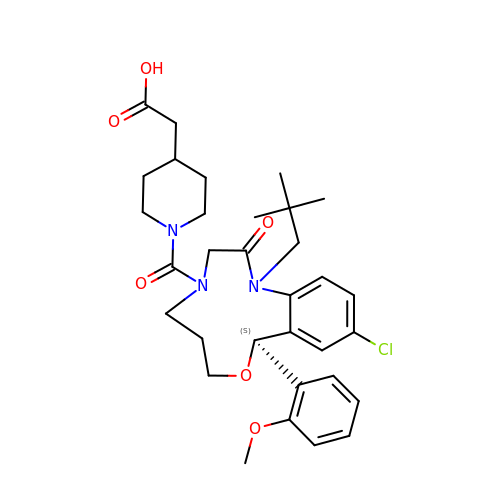2-[1-[[(10~{S})-13-chloranyl-2-(2,2-dimethylpropyl)-10-(2-methoxyphenyl)-3-oxidanylidene-9-oxa-2,5-diazabicyclo[9.4.0]pentadeca-1(15),11,13-trien-5-yl]carbonyl]piperidin-4-yl]ethanoic acid | C32 H42 Cl N3 O6 | LXTOPZNQSVXGNW-SSEXGKCCSA-N>MADLHIGNYRLLKTIGKGNFAKVKLARHILTGKEVAVKIIDKTQLNSSSLQKLFREVRIMKVLNHPNIVKLFEVIETEKTLYLVMEYASGGEVFDYLVAHGWMKEKEARAKFRQIVSAVQYCHQKFIVHRDLKAENLLLDADMNIKIADFGFSNEFTFGNKLDTFCGSPPYAAPELFQGKKYDGPEVDVWSLGVILYTLVSGSLPFDGQNLKELRERVLRGKYRIPFYMSTDCENLLKKFLILNPSKRGTLEQIMKDRWMNVGHEDDELKPYVEPLPDYKDPRRTELMVSMGYTREEIQDSLVGQRYNEVMATYLLLGY[4x];>GPVDNNNNNGLKNSTEPIYAKVNKKKTGQVASPEEPIYTQVAKKVNAKIDRLNQIASGLGGVGQAAGFPLKRHDKVD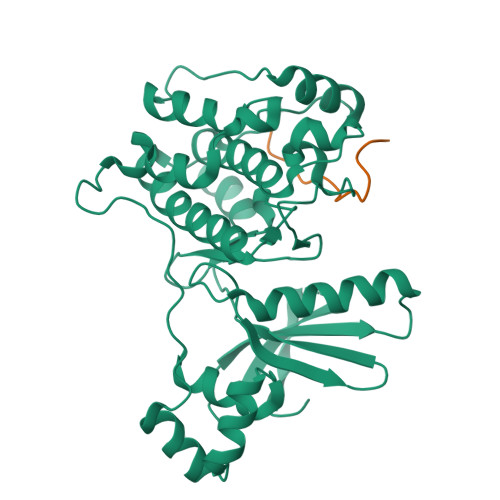DLSKVGLSASPEPIYATIDDLGGPFPLKRHDKVDDLSKVGRSRNQELA[4x]>[2x]MAQGTLYIVSA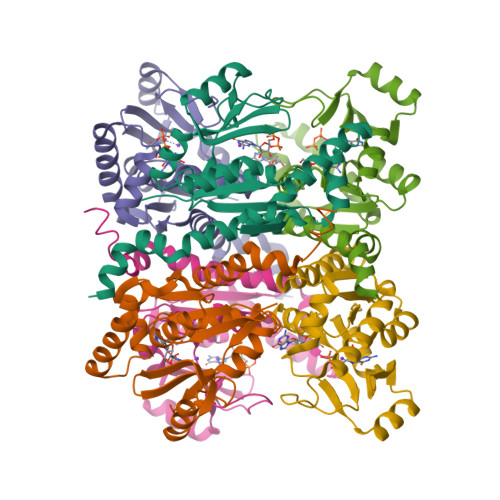PSGAGKSSLIQALLKTQPLYDTQVSVSHTTRQPRPGEVHGEHYFFVNHDEFKEMISRDAFLEHAEVFGNYYGTSREAIEQVLATGVDVFLDIDWQGAQQIRQKMPHARSIFILPPSKIELDRRLRGRGQDSEEVIAKRMAQAVAEMSHYAEYDYLIVNDDFDTALTDLKTIIRAERLRMSRQKQRHDALISKLLAD>PPPIADEPLTVNTGIYLIECYSLDDKAETFKVNAFLSLSWKDRRLAFDPVRSGVRVKTYEPEAIWIPEIRFVNVENAR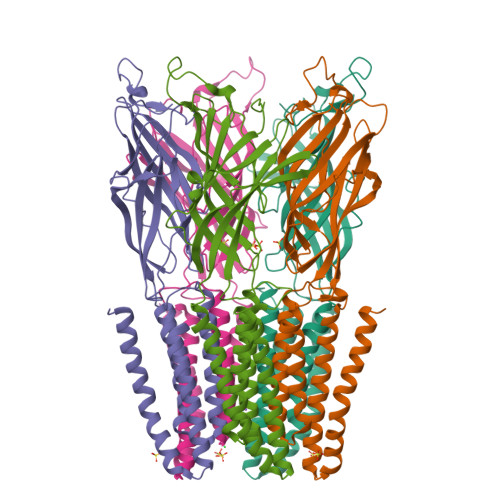DADVVDISVSPDGTVQYLERFSARVLSPLDFRRYPFDSQTLHIYLIVRSVDTRNIVLAVDLEKVGKNDDVFLTGWDIESFTAVVKPANFALEDRLESKLDYQLRISRQYFSYIPNIILPMLFILFISWTAFWSTSYIANVTLVVSTLAAHIAFNILVETNLPKTPYMTYTGAIIFMIYLFYFVAVIEVTVQHYLKVESQPARAASITRASRIAFPVVFLLANIILAFLFFGF[5x]> MSLSSWRQFQLFENIPIRDPNFGGDSLLYSDPTLCAATIVDPQTLIIAVNSNIIKVVKLNQSQVIHEFQSFPHDFQITFLKVINGEFLVALAESIGKPSLIRVYKLEKLPNREQLYHSQVELKNGNNTYPISVVSISNDLSCIVVGFINGKIILIRGDISRDRGSQQRIIYEDPSKEPITALFLNNDATACFAATTSRILLFNTTGRNRGRPSLVLNSKNGLDLNCGSFNPATNEFICCLSNFIEFFSSSGKKHQFAFDLSLRKRIFCVDKDHILIVTEETGVPTTSISVNELSPTIINRIFIIDAKNKIISLNFVVSSAIIDIFSTSQSGKNITYLLTSEGVMHRITPKSLENQINIIIQKELYPFALQLAKQHSLSPLDVQEIHKKYGDYLFKKGLRKEATDQYIQCLDVVETSEIISKFGVKEVPDPESMRNLADYLWSLIKNSISQRDHVTLLLIVLIKLKDVEGIDTFIQHFDRKGIWNEGVVMDDMDDVTFFYSDNDFFDLDLILELMKESDFKRLSYRLAKKYSKDSLIIVDILLNLLHNPVKAIKYIKSLPIDETLRCLVTYSKKLLEESPNETNALLIEVFTGKFKPSTFEVDLDRRDTTGDFSENIRTVFYSYKTFFNYMNSNGTSDAMSESSEASHEHEEPTYHPPKPSIVFSSFVTKPFEFVVFLEACLACYQQYEGFDEDRQVILTTLYDLYLNLAQNDVPERIDDWRSRATGVLRESNKLVYSAASNNTSKRVDNSIMLLISHMDQSSASAKDKTKIDIASFANDNPEMDLLSTFRAMTLNEEPSTCLKFLEKYGTEEPKLLQVALSYFVSNKLIFKEMGGNEVLKEKVLRPIIEGERMPLLDIIKALSRTNVAHFGLIQDIIIDHVKTEDTEIKRNEKLIESYDKELKEKNKKLKNTINSDQPLHVPLKNQTCFMCRLTLDIPVVFFKCGHIYHQHCLNEEEDTLESERKLFKCPKCLVDLETSNKLFEAQHEVVEKNDLLNFALNSEEGSRDRFKVITEFLGRGAISYSDITI;> MKNPSFDWERLKDVFYRSRAIGELKWPTQYEEFKCALSLTVIAVEIQDFIQVYNYFGQLLGKINLQRIHEDIIKFEFDKDEKLILVTKSSIKIVKGWSPLTIESVPLQDPTIDTIWDYHNGIMLLAKSRDIYKLNGNEWELLYENKDKKYNLLTKNHWSCNDDSIILLDVDHVYQVSTSNGALLKLITDSSWHKVTISSRGFICLYNMKDNKLQIFRDPARILMEHNLDSTPDDICWCGNDTVACSFEDEIKLYGPDGLYVTFWYPFTVTNLRAEVDGLKVITTEKIYFLSRVQPQTSNIFRIGSTEPGAMLVDSFSLLEDHAPKAIEILKNFVLEKGVLDCIAAAIDEFEPKLQKMLLNAASYGKASLQYKSFDASIFVNACNTIKLLNCFRSFGIFLTVEEYRCISLKGVIDRLLKYHRYYECIQICKLANERFLLGYVFTEWAKDKIKGSPDMEDDELLDKIKSRLSVIDMTDTLQMVAVAKVAYLEGRFQLSRNLALLEKNEEARIEQLYNLDDDSIALKECIKVQNYSLTISLLIALSKKLTNSQLTKLLIIDMFNNPLYLYYMRMDKAYLYDFYRQTDRFIDLAHVLLQQGKEQQSLHSFLPQIKDLYSQVQNSEVVNNTIEQLQRQEKLWIYQESLGKRFAISFTNMTLDQTLSKLIETGQDKQVKEIVKKFKISEKKLYHLKCKTLVEAKKFDELLQFAQSRKSPIGYMPFYTYLKSRGHMDKASPYVNMIPGLSYQEKKKLYVECRGFRDAIQLAGKEKDIPGLKEIYNIIPPNEPELKALANETMSRI;> MIKTRIEEVQLQFLTGNTELTHLKVSNDQLIVTTQRTIYRINLQDPAIVNHFDCPLSKELETIMNVHVSPMGSVILIRTNFGRYMLLKDGEFTQLNKIKNLDLSSLHWINETTFLMGIKKTPKLYRVELTGKDITTKLWYENKKLSGGIDGIAYWEGSLLLTIKDNILYWRDVTNMKFPLVLPDESEQFERLKHHAIKKFDSYNGLFAWVTSNGIVFGDLKEKQMEKDPASNNFGKFLSSSKVLLNFELPDYQNDKDHLIKDIVLTAFHILLLRKNTVTMVSQLNNDVVFHETIPRHQLTGSNTDSNEKFLGLVRDSVKETFWCFSNINVFEIIIENEPNSVWNLLVRDNKFDKALSLKGLTVREIESVKLSKAMYLFHTAKDFHSAAQTLGSMKDLSHFGEIALNFLQIKDYNDLNVILIKQLDNVPWKSTQVVLSSWIIWNFMKQLNDIELKINTTKPASTDEDNLLNWNLNLKEKSNELTKFLESHLEKLDNETVYQIMSKQNRQNELLIFASLINDMKFLLSFWIDQGNWYESLKILLTINNHDLVYKYSLILLLNSPEATVSTWMKIKDLDPNKLIPTILKFFTNWQNNSKLITNISEYPENYSLTYLKWCVREVPKMCNPIVYNSILYMMITDPRNDMILENDIIKFMKSNENKYDLNFQLRLSLKFKKTKTSIFLLTRLNLFEDAIDLALKNNLIDDCKVIVNDEILIEDYKLRKRLWLKIAKHLLLSMKDIDIKQLIRTILNDSNEILTIKDLLPFFNEYTTIANLKEELIKFLENHNMKMNEISEDIINSKNLKVEINTEISKFNEIYRILEPGKSCDECGKFLQIKKFIVFPCGHCFHWNCIIRVILNSNDYNLRQKTENFLKAKSKHNLNDLENIIVEKCGLCSDININKIDQPISIDETELAKWNE;> MNRFWNTKKFSLTNADGLCATLNEISQNDEVLVVQPSVLPVLNSLLTFQDLTQSTPVRKITLLDDQLSDDLPSALGSVPQMDLIFLIDVRTSLRLPPQLLDAAQKHNLSSLHIIYCRWKPSFQNTLEDTEQWQKDGFDLNSKKTHFPNVIESQLKELSNEYTLYPWDLLPFPQIDENVLLTHSLYNMENVNMYYPNLRSLQSATESILVDDMVNSLQSLIFETNSIITNVVSIGNLSKRCSHLLKKRIDEHQTENDLFIKGTLYGERTNCGLEMDLIILERNTDPITPLLTQLTYAGILDDLYEFNSGIKIKEKDMNFNYKEDKIWNDLKFLNFGSIGPQLNKLAKELQTQYDTRHKAESVHEIKEFVDSLGSLQQRQAFLKNHTTLSSDVLKVVETEEYGSFNKILELELEILMGNTLNNDIEDIILELQYQYEVDQKKILRLICLLSLCKNSLREKDYEYLRTFMIDSWGIEKCFQLESLAELGFFTSKTGKTDLHITTSKSTRLQKEYRYISQWFNTVPIEDEHAADKITNENDDFSEATFAYSGVVPLTMRLVQMLYDRSILFHNYSSQQPFILSREPRVSQTEDLIEQLYGDSHAIEESIWVPGTITKKINASIKSNNRRSIDGSNGTFHAAEDIALVVFLGGVTMGEIAIMKHLQKILGKKGINKRFIIIADGLINGTRIMNSIS;> MLRAQKLHSLKSSDITAILPTEQSQKLVLAKKNGDVEVYSRDGNTLKLFQVYPDLLQNAKNDPLPPVIENFYFANELSTIFAQCKETLILLSTTNLHEYDRIIDRRGINHCWLFERSHKNKEEKNTYLIYSTINTAKMRVLIWEGRTYKNMMEASLSYRKETIRSIYPGETGITLATDLGIYHWPYNKPSLIRIEKTVKNKFPKDMISALTELKEQAEKVIEKKPKKNSHFDAQSFSSMDRMSRKSSMSSLWYRTIRNERGNKIRYTFELDGNDATPMIIDGATKKIFKVELMHNNEEPFLIATDHATFSESNSEFDHMQYLSSNLLMLYNSSTIKFVDYENGFTFLQQKIPEGIKWVKNLSGTYFLVWTSNDEVQLFSYHVDDGSEDDDQESICGDINDPDFYQLWRKVLFYKFFIDSPHSKELCVSDNPEESLDICAMKLRDLTVMWCLRIFDKFQNYMVQLERSRNSRMIRSKCEEMIIKSIFDLFIKFWAPPQLVILKVFPSAISSLVLEITGQEHHCLLKEAEEVKETYDIPPHLLNRWCLPYLTDTRRHLQNLLSKENDDESRITWCYRDREIKQSFDFFLISNHDDVDLNTMLTLIDTVLFKCYLYYNPPMVGPFIRVENHCDSHVIVTELKIRHMFKDLIDFYYKRGNHEEALKFLTDLVDELENDNTDQKQRQKIDHGVKILVIYYLKKLSNPQLDVIFTYTDWLLNRHNDSIKEILSSIFFYDSQACSSRDHLKVYGYIKKFDKLLAIQYLEFAISTFRLEGNKLHTVLIKLYLENLDIPSTRIKLKSLLETTSVYEPRTILKLLNDAIESGSDQLPTNQLNFVKYLKIFPLSKLENHKEAVHILLDEIDDYKAATSYCNDVYQSDSTKGEELLLYLYSKLVSIYDSNRNSKLILNFLQDHGSKLNSAEIYKNLPQDISLYDIGRVVSQLLKKHTSKMDETRLEKALLQVELVATTYKLNERMSSYGVLSDSHKCPICKKVISNFGTDSISWFTREGRNIITHYNCGKVLQERFNAKNEKSSRIKQKTLGEVINELNNK;> MTTDNHQNDSVLDQQSGERTIDESNSISDENNVDNKREDVNVTSPTKSVSCISQAENGVASRTDESTITGSATDAETGDDDDDDDDDDDEDEDDEDEPPLLKYTRISQLPKNFFQRDSISSCLFGDTFFAFGTHSGILHLTTCAFEPIKTIKCHRSSILCINTDGKYFATGSIDGTVIIGSMDDPQNITQYDFKRPINSVALHSNFQASRMFVSGGMAGDVVLSQRNWLGNRIDIVLNKKKKKKTRKDDLSSDMKGPIMGIYTMGDLILWMDDDGITFCDVPTRSQLLNIPFPSRIFNVQDVRPDLFRPHVHFLESDRVVIGWGSNIWLFKVSFTKDSNSIKSGDSNSQSNNMSHFNPTTNIGSLLSSAASSFRGTPDKKVELECHFTVSMLITGLASFKDDQLLCLGFDIDIEEEATIDEDMKEGKNFSKRPENLLAKGNAPELKIVDLFNGDEIYNDEVIMKNYEKLSINDYHLGKHIDKTTPEYYLISSNDAIRVQELSLKDHFDWFMERKQYYKAWKIGKYVIGSEERFSIGLKFLNSLVTKKDWGTLVDHLNIIFEETLNSLDSNSYDVTQNVLKEWADIIEILITSGNIVEIAPLIPKKPALRKSVYDDVLHYFLANDMINKFHEYITKWDLKLFSVEDFEEELETRIEAASEPTASSKEEGSNITYRTELVHLYLKENKYTKAIPHLLKAKDLRALTIIKIQNLLPQYLDQIVDIILLPYKGEISHISKLSIFEIQTIFNKPIDLLFENRHTISVARIYEIFEHDCPKSFKKILFCYLIKFLDTDDSFMISPYENQLIELYSEYDRQSLLPFLQKHNNYNVESAIEVCSSKLGLYNELIYLWGKIGETKKALSLIIDELKNPQLAIDFVKNWGDSELWEFMINYSLDKPNFTKAILTCSDETSEIYLKVIRGMSDDLQIDNLQDIIKHIVQENSLSLEVRDNILVIINDETKKFANEFLKIRSQGKLFQVDESDIEINDDLNGVLDYKDDDDKDYKDDDDKDYKDDDDK

Lysosomal fusion is fundamental to cell survival and requires HOPS, a conserved heterohexameric tethering complex. The heterohexameric HOPS complex mediates fusion of late endosomes, autophagosomes, and AP-3 vesicles with mammalian lysosomes or vacuoles in yeast, and is probably the best-studied tethering complex. Five out of six HOPS subunits (Vps11, Vps16, Vps18, Vps39, and Vps41) are predicted to share a similar architecture, comprising an N-terminal β-propeller and a C-terminal α-solenoid domain. At the opposite sites, Vps41 and Vps39 bind to membrane-anchored small GTPases (the Rab7-like Ypt7 in yeast), while Vps16 and the SM protein Vps33 establish the SNARE-binding module.

Here, we used cryo-electron microscopy to reveal the structure of HOPS. To enable high-resolution cryo-EM of non-crosslinked HOPS, we vastly improved and accelerated our purification protocols and removed any delays during the sample preparation procedure. Single-particle analysis including extensive classifications followed by local refinements led to a composite structure with resolutions between 3.6 and 5 Å (Figure 1E and Figure 1—figure supplements 1–3). HOPS forms a largely extended, slender structure extending approximately 430 Å in height and 130 Å in width, resembling a triangular shape. In the center of the modular complex, Vps11 and Vps18 align antiparallel through their elongated α-solenoids, establishing a large interface area of 1972 Å2, which resulted in the highest resolution obtained within HOPS and is comparable with protein interfaces in other complexes with similar structural elements as in HOPS. In our model, the two core subunits create a central assembly hub for the four other subunits (Vps39, Vps41, Vps16, and Vps33) that fulfill specific functions and localize to the periphery of the complex. Vps41 and Vps39 provide the Ypt7-interaction sites at their peripheral N-terminal regions. Their extended C-terminal helices, similar to those of Vps11 and Vps18, are tightly interlocked through coiled-coil motifs with the long C-terminal α-helices and RING finger domains from the respective core subunits (Vps41 with Vps18, and Vps39 with Vps11). Vps33 is in immediate contact with the structured loop of Vps18 (residues 824–831) that connects the elongated helix with the RING finger domain. Overall, the SNARE binding module appears to be stably connected to the central core, while only the short C-terminal section of Vps16 α-solenoid (residues 739–798) displays high variability and is not resolved in our structure. Multi-modular classification analyses revealed angular re-orientations of about 9° for Vps41 and 20° for Vps39 relative to the core, resulting in variable positions of the N-terminal β-propellers.>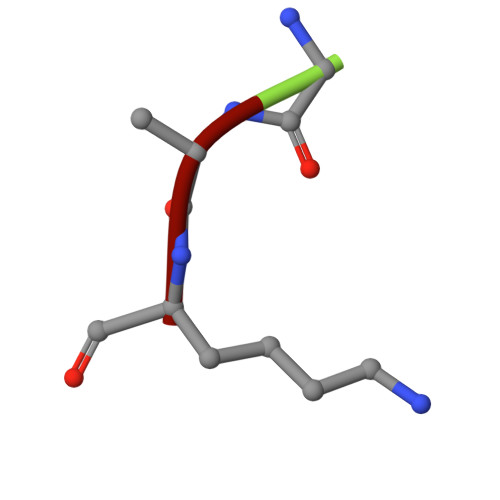 GAK> PNFSGNWKIIRSENFEELLKVLGVNVMLRKIEVAAASKPAVEIKQEGDTFYIKTSTTVRTTEINFKVGEEFEEQT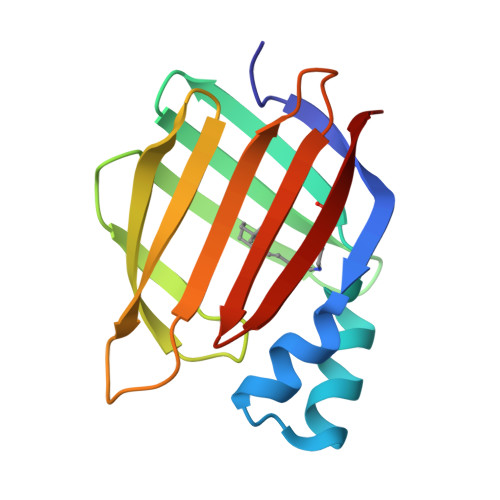VDGRPCKSLVKWESENKMVCEQKLLKGEGPKTSWTLELTNDGELILTMTADDVVCTKVYVRE N-[4,5-BIS(4-HYDROXYPHENYL)-1,3-THIAZOL-2-YL]HEXANAMIDE 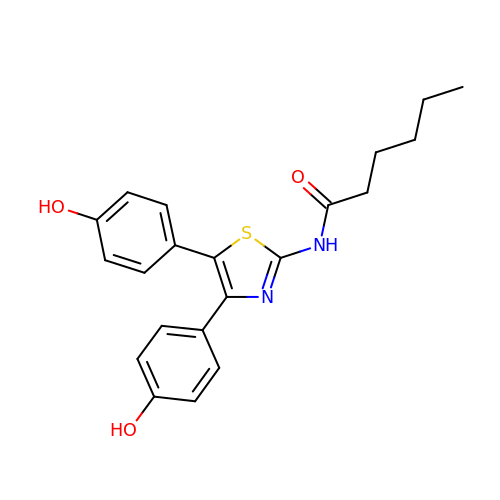| C21 H22 N2 O3 S | RPLGSGRXKXSQAO-UHFFFAOYSA-N> VEKLTADAELQRLKNERHEEAELERL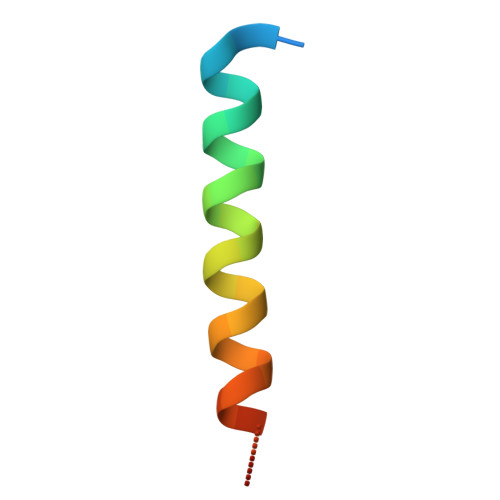LSEY>[2x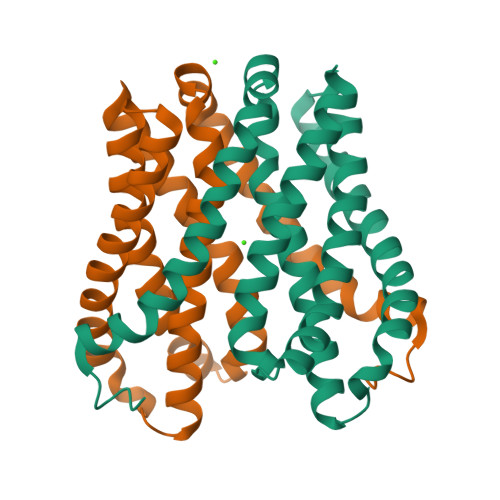]LVYSEAGPVALWLARVRWLVILILTGMVTSSILQGFESVLEAVTALAFYVPVLLGTGGNTGNQSATLIIRALATRDLDLRDWRRVFLKEMGVGLLLGLTLSFLLVGKVYWDGHPLLLPVVGVSLVLIVFFANLVGAMLPFLLRRLGVDPALVSNPLVATLSDVTGLLIYLSVARLLLE> GMTEIVKASLENGIQKIRIQAEKGYHPAHIQLQKGIPAEIT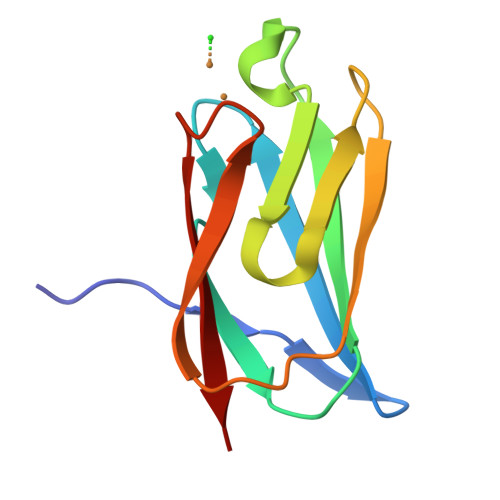FHRATPSNCYKEILFEEEGILEPIGVDEEKVIRFTPQELGRHEFSCGMKMQKGSYTVVE> LDARQFLIYNEDHKRCVDALSAISVQTATCNPEAESQKFRWVSDSQIMSVAFKLCLGVPSKT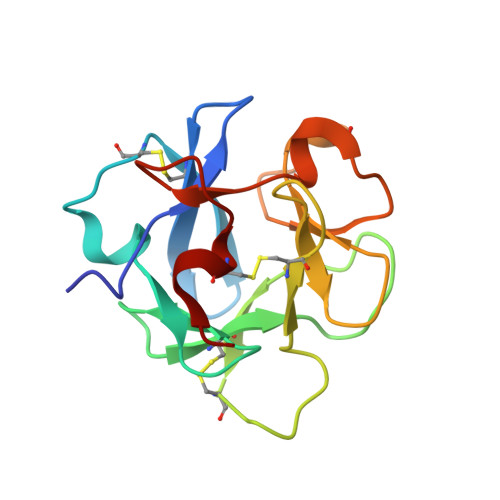DWASVTLYACDSKSEYQKWECKNDTLFGIKGTELYFNYGNRQEKNIKLYKGSGLWSRWKVYGTTDDLCSRGYE> EDVEIKPRGYQLRLVDHLTKSNGIVYLPTGSGKTFVAILVLKRFSQDFDKPIESGGKRALFMCNTVELARQQAMAVRRCTNFKVGFYVGEQGVDDWTRGMWSDEIKKNQVLVGTAQVFLDMVTQTYVALSSLSVVIIDECHHGTGHHPFREFMRLFTIANQTKLPRVVGLTGVLIKGNEITNVATKLKELEITYRGNIITVSDTKEMENVMLYATKPTEVMVSFPHQEQVLTVTRLISAEIEKFYVSLDLMNIGVQPIRRSKSLQCLRDPSKKSFVKQLFNDFLYQMKEYGIYAASIAIISLIVEFDIKRRQAETLSVKLMHRTALTLCEKIRHLLVQKLQDMTYDDDDDNVNTEEVIMNFSTPKVQRFLMSLKVSFADKDPKDICCLVFVERRYTCKCIYGLLLNYIQSTPELRNVLTPQFMVGRNNISPDFESVLERKWQKSAIQQFRDGNANLMICSSVLEEGIDVQACNHVFILDPVKTFNMYVQSKGRARTTEAKFVLFTADKEREKTIQQIYQYRKAHNDIAEYLKDRVLEKTEPELYEIKGHFQDDIDPFTNENGAVLLPNNALAILHRYCQTIPTDAFGFVIPWFHVLQEDERDRIFGVSAKGKHVISINMPVNCMLRDTIYSDPMDNVKTAKISAAFKACKVLYSLGELNERFVPKTLKERVASIADVHFEHWNKYGDSVTATVNKADKSKDRTYKTECPLEFYDALPRVGEICYAYEIFLEPQFESCEYTEHMYLNLQTPRNYAILLRNKLPRLAEMPLFSNQGKLHVRVANAPLEVIIQNSEQLELLHQFHGMVFRDILKIWHPFFVLDRRSKENSYLVVPLILGAGEQKCFDWELMTNFRRLPQSHGSNVQQREQQPAPRPEDFEGKIVTQWYANYDKPMLVTKVHRELTPLSYMEKNQQDKTYYEFTMSKYGNRIGDVVHKDKFMIEVRDLTEQLTFYVHNRGKFNAKSKAKMKVILIPELCFNFNFPGDLWLKLIFLPSILNRMYFLLHAEALRKRFNTYLNLHLLPFNGT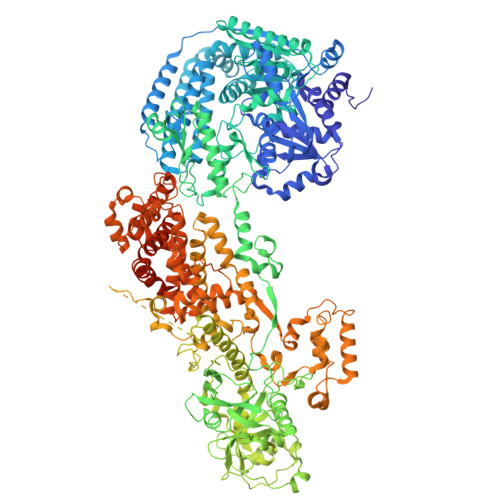DYMPRPLEIDYSLKRNVDPLGNVIPTEDIEEPKSLLEPMPTKSIEASVANLEITEFENPWQKYMEPVDLSRNLLSTYPVELDYYYHFSVGNVCEMNEMDFEDKEYWAKNQFHMPTGNIYGNRTPAKTNANVPALMPSKPTVRGKVKPLLILQKTVSKEHITPAEQGEFLAAITASSAADVFDMERLEILGNSFLKLSATLYLASKYSDWNEGTLTEVKSKLVSNRNLLFCLIDADIPKTLNTIQFTPRYTWLPPGISLPHNVLALWRENPEFAKIIGPHNLRDLALGDEESLVKGNCSDINYNRFVEGCRANGQSFYAGADFSSEVNFCVGLVTIPNKVIADTLEALLGVIVKNYGLQHAFKMLEYFKICRADIDKPLTQLLNLELGGKKMRANVNTTEIDGFLINHYYLEKNLGYTFKDRRYLLQALTHPSYPTNRITGSYQELEFIGNAILDFLISAYIFENNTKMNPGALTDLRSALVNNTTLACICVRHRLHFFILAENAKLSEIISKFVNFQESQGHRVTNYVRILLEEADVQPTPLDLDDELDMTELPHANKCISQEAEKGVPPKGEFNMSTNVDVPKALGDVLEALIAAVYLDCRDLQRTWEVIFNLFEPELQEFTRKVPINHIRQLVEHKHAKPVFSSPIVEGETVMVSCQFTCMEKTIKVYGFGSNKDQAKLSAAKHALQQLSKCDA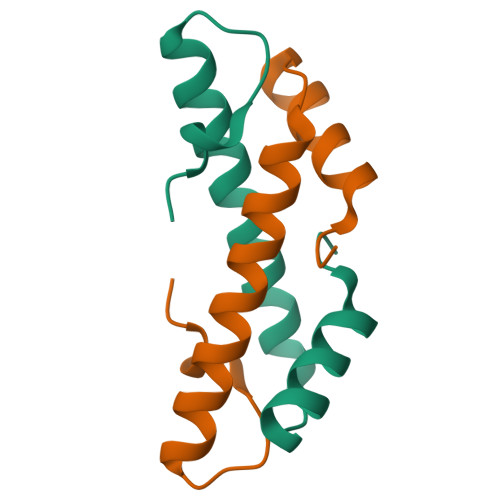> GHMAEVLVVTSKVKKLIKEKGQMNTSAETIDVLSKAIEQLCLKGVESAKADGRKTVMARDIVIDHL>[2x]MRPSDAWPRHSAERRPWAQTQRGGTRADRTLRSVTVSLPPYIAKVDANIDADIAVKLEDAMSEISRLDSTHGTHLAGLSTLLLRTESVASSKIERVEASVDDYARALHGGRGNSSAVSMVAATTALKEMIASVNRDAPI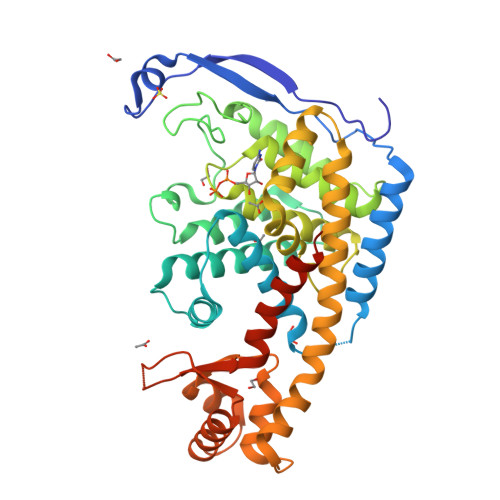QMTAILRAHEALMREDPTEGQHAGQVRTVQNWIGGSDYSPRNALYVPPPPDTVHAYMDDLIEFANRTDIPVLIQAAIAHAQFESIHPFTDGNGRIGRALINTVLRRRGATTRLVVPLASALVAHRERYFGALNTYRAGDLRPLIVTFANSSRTAAAESRITAERLAEIPVEWRNMVGPIRRHSATDKLLLLLPSTPIVSSDDVASLIDAPRSSVFAAIKRLHDTGVLRPLTNRKRDQVWGASLVLDELDDLGHRIERASAPSVRKLEHHHHHH> PDQFRAIIESPEGAGHVGYQYRRNTGSTMRMVSDVLDERVSLWDFHCDPSGNVIQPGPNVDSRQYLQAAIDYVSSNGGGTITIPAGYTWYLGSYGVGGIAGHSGIIQLRSNVNLNIEGRIHLSPFFDLKPFQV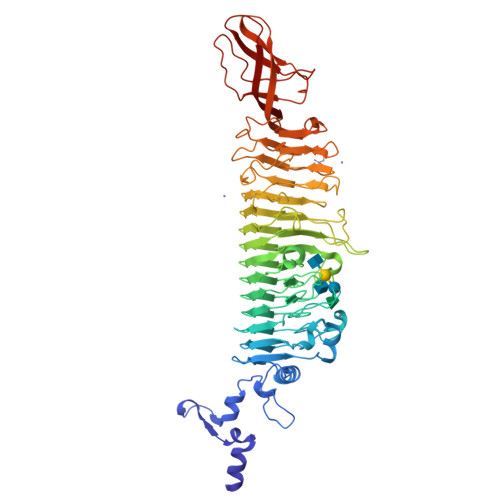FVGFDNGDPASSGNLENCHIYGHGVVDFGGYEFGASSQLRNGVAFGRSYNCSVTGITFQNGDVTWAITLGWNGYGSNCYVRKCRFINLVNSSVNADHSTVYVNCPYSGVESCYFSMSSSFARNIACSVELHQHDTFYRGSTVNGYCRGAYVVMHAAEAAGAGSYAYNMQVENNIAVIYGQFVILGSDVTATVSGHLNDVIVSGNIVSIGERAAFSAPFGAFIDIGPDNSGASNVQDIQRVLVTGNSFYAPANITDSAAITLRANLNGCTFIANNFDCRYMVYNAPGTTSPVVQNLVWDKSNVIGGTHANQRAGQNLFDMQFASVVNSTIEVQLSCEDLSMFSCILFPASCQLSYSKITVDSAWTKSMSNTAVFEGNQQAGANVYVSYPATVNLTSYNTQGAVPFFSTDTNYAWVTSAYSLSINENLDFSPPATYTNKANGQLVGVGYNEIGGVRSVSVRLMLQRQV> PEIGNNGAEKQISLHKGQPFIDTQDVGAADPNTPAVTIEGPSDYVIAIDAGTPVAPEFRDANGDKLDPSTRVTIQKCDKQGN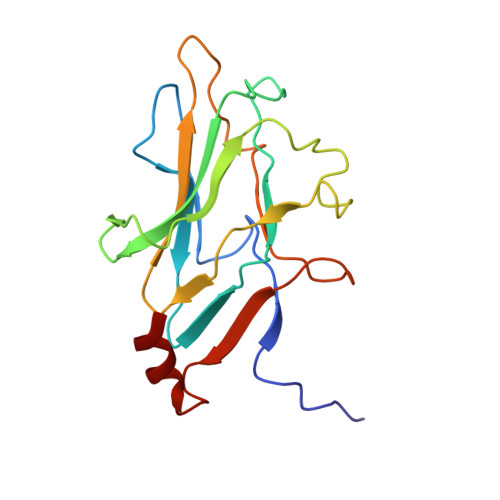PLGDGIVFSDTLGRFEYSKMRSDPDYMRKTTTSLMIDEREIVKIFVEVPPNANGMDADNSRITIGDDTSDYGKAVGIVEHGDLSPAESKAVRQ> GADDVVDSSKSFVMENFSSYHGTKPGYVDSIQKGIQKPKSGTQGNYDDDWKGFYS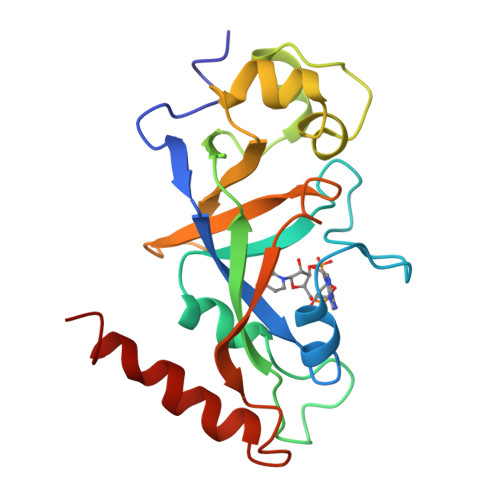TDNKYDAAGYSVDNENPLSGKAGGVVKVTYPGLTKVLALKVDNAETIKKELGLSLTEPLMEQVGTEEFIKRFGDGASRVVLSLPFAEGSSSVEYINNWEQAKALSVELEINFETRGKRGQDAMYEYMAQACAGNR> MADSQPLSGAPEGAEYLRAVLRAPVYEAAQVTPLQKMEKLSSRLDNVILVKREDRQPVHSFKLRGAYAMMAGLTEEQKAHGVITASAGN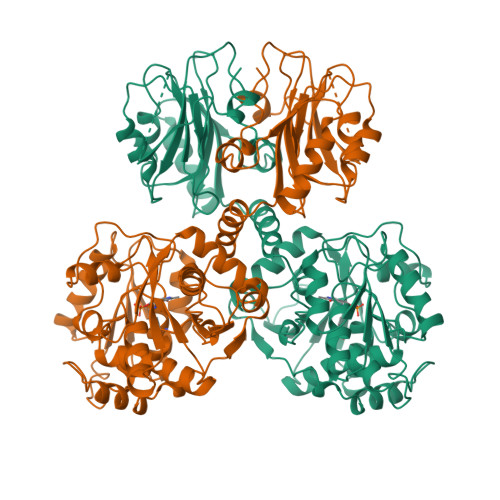HAQGVAFSSARLGVKALIVMPTATADIKVDAVRGFGGEVLLHGANFDEAKAKAIELSQQQGFTWVPPFDHPMVIAGQGTLALELLQQDAHLDRVFVPVGGGGLAAGVAVLIKQLMPQIKVIAVEAEDSACLKAALDAGHPVDLPRVGLFAEGVAVKRIGDETFRLCQEYLDDIITVDSDAICAAMKDLFEDVRAVAEPSGALALAGMKKYIALHNIRGERLAHILSGANVNFHGLRYVSERCELGEQREALLAVTIPEEKGSFLKFCQLLGGRSVTEFNYRFADAKNACIFVGVRLSRGLEERKEILQMLNDGGYSVVDLSDDEMAKLHVRYMVGGRPSHPLQERLYSFEFPESPGALLRFLNTLGTYWNISLFHYRSHGTDYGRVLAAFELGDHEPDFETRLNELGYDCHDETNNPAFRFFLAG GLUTATHIONE 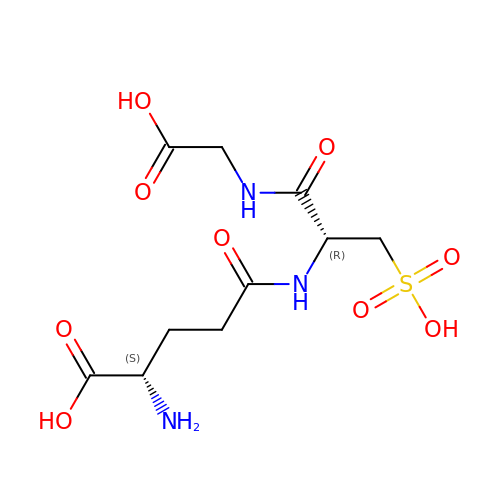SULFONIC ACID | C10 H17 N3 O9 S | QGWRMTHFAZVWAM-WDSKDSINSA-N>TRDRVPTYQYNMNFEKLGKCIIINNKNFDKVTGMGVRNGTDKDAEALFKCFRSLGFDVIVYNDCSCAKMQDLLKKASEEDHTNAACFACILLSHGEENVIYGKDGV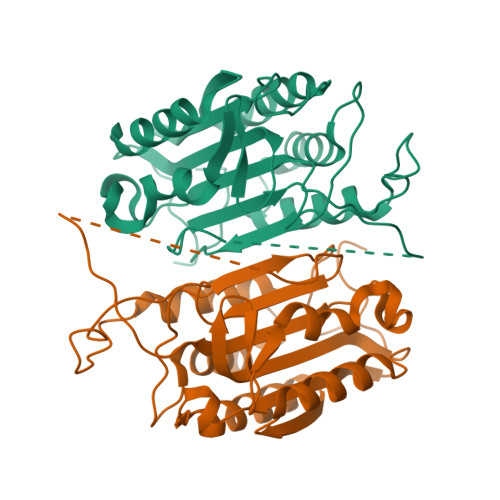TPIKDLTAHFRGARCKTLLEKPKLFFIQACRGTELDDGIQADSGPINDTDANPRYKIPVEADFLFAYSTVPGYYSWRSPGRGSWFVQALCSILEEHGKDLEIMQILTRVNDRVARHFESQSDDPHFHEKKQIPCVVSMLTKELYFSQ[2x]3-decanoyloxypropyl decanoate | C23 H44 O4 | 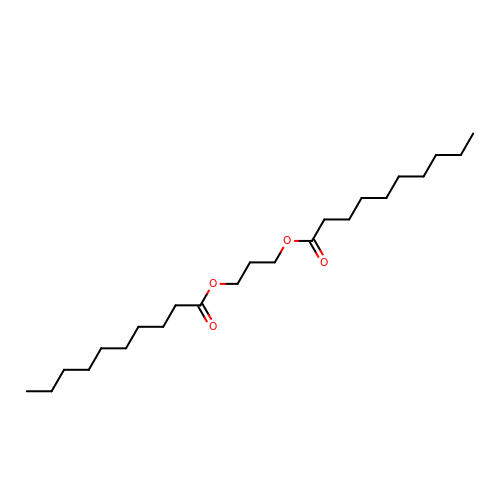PXVAQENAIBBOHT-UHFFFAOYSA-N> MIRTMLQGKLHRVKVTHADLH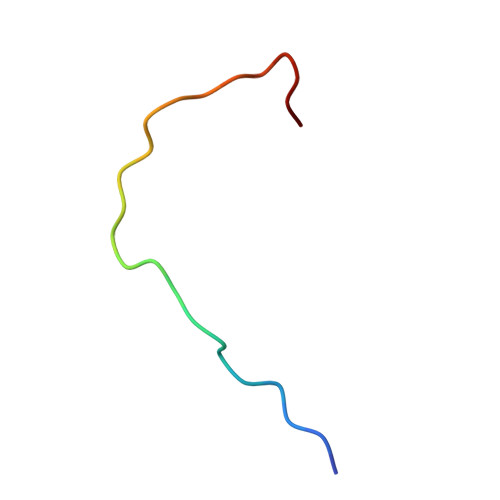YEG>[12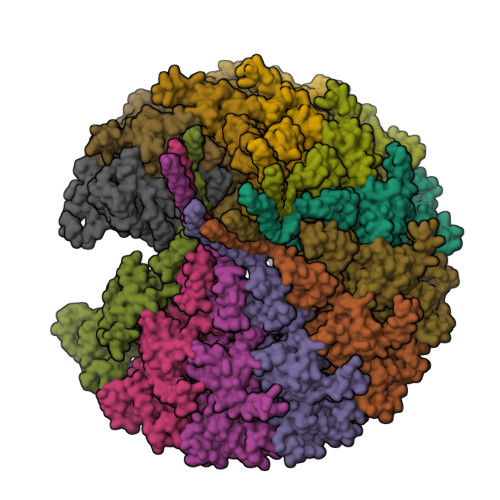x]MAKRRKIKPMDDEQVLRHLDQLVNDALDFNSSELSKQRSEALKYYFGEPFGNERPGKSGIVSRDVQETVDWIMPSLMKVFTSGGQVVKYEPDTAEDVEQAEQETEYVNYLFMRKNEGFKVMFDWFQDTLMMKTGVVKVYVEEVLKPTFERFSGLSEDMVADILSDPDTSILAQSVDDDGTYTIKIRKDKKKREIKVLCVKPENFLVDRLATCIDDARFLCHREKYTVSDLRLLGVPEDVIEELPYDEYEFSDSQPERLVRDNFDMTGQLQYNSGDDAEANREVWASECYTLLDVDGDGISELRRILYVGDYIISNEPWDCRPFADLNAYRIAHKFHGMSVYDKIRDIQEIRSVLMRNIMDNIYRTNQGRSVVLDGQVNLEDLLTNEAAGIVRVKSMNSITPLETPQLSGEVYGMLDRLEADRGKRTGITDRTRGLDQNTLHSNQAAMSVNQLMTAAEQQIDLIARMFAETGVKRLFQLLHDHAIKYQNQEEVFQLRGKWVAVNPANWRERSDLTVTVGIGNMNKDQQMLHLMRIWEMAQAVVGGGGLGVLVSEQNLYNILKEVTENAGYKDPDRFWTNPNSPEALQAKAIREQKEAQPKPEDIKAQADAQRAQSDALAKQAEAQMKQVEAQIRLAEIELKKQEAVLQQREMALKEAELQLERDRFTWERARNEAEYHLEATQARAAYIGDGKVPETKKPTKAVRR>[2x]MGEPRSQPPVERPPTAETFLPLSRVRTIMKSSMDT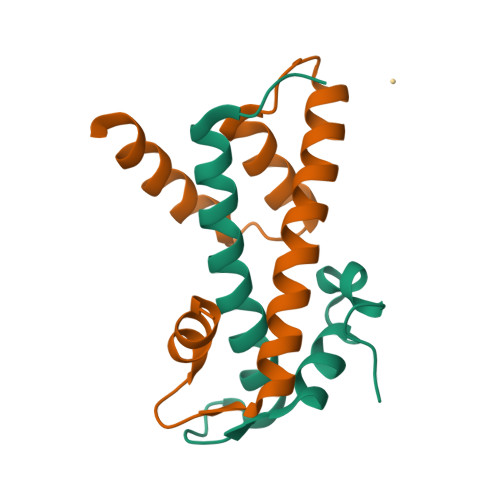GLITNEVLFLMTKCTELFVRHLAGAAYTEEFGQRPGEALKYEHLSQVVNKNKNLEFLLQIVPQKIRVHQFQEMLRLNRSAGSDDDDDDDDDDDEEESESESESDE;>[2x]MVERIEDLNLPNAVIGRLIKEALPESASVSKEARAAIARAASVFAIFVTSSSTALAHKQNHKTITAKDILQTLTELDFESFVPSLTQDLEVYRKVVKEKKESKASKKDSNTAENANASATATAEEAPE>[2x]SMKEWQENKSWNAHFTEHKSQGVVVLWNENKQQGFTNNLKRANQAFLPASTFKIPNSLIALDLGVVKDEHQVFKWDGQTRDIATWNRDHNLITAMKYSVVPVYQEFARQIGEARMSKMLHAFDYGNEDISGNVDSFWLDGGIRISATEQISFLRKLYHNKLHVSERSQRIVKQAMLTEANGDYIIRAKTGYSCRIEPKIGWWVGWVELDDNVWFFAMNMDMPTSDGLGLRQAITKEVLKQEKIIP

The active sites of class D carbapenemases such as OXA‐48, which is of major clinical importance, uniquely contain a carbamylated lysine residue which is essential for catalysis. Unlike other classes of SBLs, class D catalysis requires carbamylation of a lysine residue, which occurs through the reversible reaction of carbon dioxide/bicarbonate with the lysine ϵ‐amino group. We report the application of 19F NMR spectroscopy to investigate carbamylation of the class D SBL OXA‐48, a major clinical cause of carbapenem resistance. Crystallographic studies on 19F‐labelled OXA‐48 provide a structural rationale for the sensitivity of the 19F label to active site interactions.

We anticipated that a 19F label situated near the active site of OXA‐48, which has no cysteine residues in its wild‐type sequence, would be sensitive to its carbamylation state, so enabling the factors influencing this post‐translational modification to be investigated by 19F NMR spectroscopy. Thr213, which is positioned on the β5‐β6 loop, is poorly conserved among class D SBLs. As OXA‐48 T213C* was judged to more closely resemble the wild‐type enzyme (although, as noted, the 19F‐labelling did apparently impact kinetic behaviour), it was chosen for subsequent 19F NMR studies. Notably, unlike our crystal structure of 1,1,1‐trifluoroacetone (TFA)‐labelled metallo‐β‐lactamase SPM‐1,18 clear electron density representing the TFA label was observed in the OXA‐48 T213C* structure. The trifluoroacetone label is present in its hydrated (diol) form in the crystalline state. Hence, our 19F NMR studies in solution likely represent, at least normally, the hydrated state of the TFA label. Comparison of the OXA‐48 T213C* structure with the structure of a carbapenem‐derived OXA‐48 acyl‐enzyme complex implies the overlap of the TFA label and elements of the carbapenem acyl‐enzyme complex. Consequently, the 19F label must be displaced from this position following substrate or inhibitor binding, as manifested by changes in the 19F NMR spectrum (3 C). The presence of the 19F label in OXA‐48 T213C* close to the active site likely causes the observed changes in kinetic properties when compared to wild‐type OXA‐48. However, since these differences are relatively minor, and as the carbamylation of the 19F‐labelled enzyme behaves similarly to what was previously observed for wild‐type OXA‐48,5 the presence of the label does not appear to have a major impact on carbamylation and enzymatic activity, suggesting that the positioning of the label in OXA‐48 T213C* is dynamic, and does not obstruct access to the active site.>[3x]SMHLICQSGDVLSARYEIVDTLGEGAFGKVVECIDHKAGGRHVAVKIVKNVDRYCEAARSEIQVLEHLNTTDPNSTF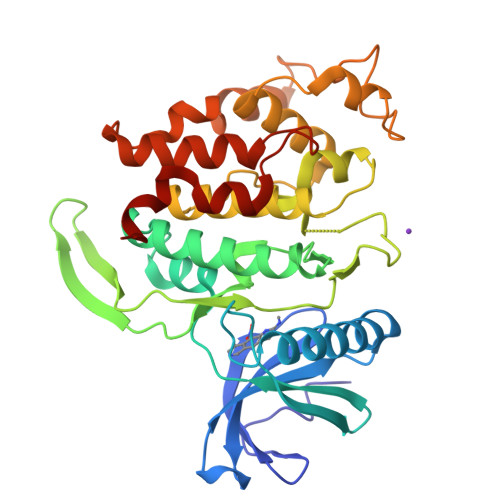RCVQMLEWFEHHGHICIVFELLGLSTYDFIKENGFLPFRLDHIRKMAYQICKSVNFLHSNKLTHTDLKPENILFVQSDYTEAYNPKIKRDERTLINPDIKVVDFGSATYDDEHHSTLVSTRHYRAPEVILALGWSQPCDVWSIGCILIEYYLGFTVFPTHDSKEHLAMMERILGPLPKHMIQKTRKRKYFHHDRLDWDEHSSAGRYVSRACKPLKEFMLSQDVEHERLFDLIQKMLEYDPAKRITLREALKHPFFDLLKKSI> GFTDYKVADITLAAWGRRELIIAESEMPALMGLRRKYAGQQPLKGAKILGCIHMTIQTGVLIETLVALGAEVRWSSCNIFSTQDQAAAAIAAAGIPVFAWKGETEEEYEWCIEQTILKDGQPWDANMVLDDGGDLTEILHKKYPQMLERIHGITEETTTGVHRLLDMLKNGTLKVPAINVNDSVTKSKNDNKYGCRHSLNDAIKRGTDHLLSGKQALVIGYGDVGKGSSQSLRQEGMIVKVAEVDPICAMQACMDGFEVVSPYKNGINDGTEASIDAALLGKIDLIVTTTGNVNVCDANMLKALKKRAVVCNIGHFDNEIDTAFMRKNWAWEEVKPQVHKIHRTGKDGFDAHNDDYLILLAEGRLVNLGNATGHPSRIMDGSFANQVLAQIHLFEQKYADLPAAEKAKRLSVEVLPKKLDEEVALEMVKGFGGVVTQLTPKQAEYIGVSVEGPFKPDTYRY;>[3x]FTDYKVADITLAAWGRRELIIAESEMPALMGLRRKYAGQQPLKGAKILGCIHMTIQTGVLIETLVALGAEVRWSSCNIFSTQDQAAAAIAAAGIPVFAWKGETEEEYEWCIEQTILKDGQPWDANMVLDDGGDLTEILHKKYPQMLERIHGITEETTTGVHRLLDMLKNGTLKVPAINVNDSVTKSKNDNKYGCRHSLNDAIKRGTDHLLSGKQALVIGYGDVGKGSSQSLRQEGMIVKVAEVDPICAMQACMDGFEVVSPYKNGINDGTEASIDAALLGKIDLIVTTTGNVNVCDANMLKALKKRAVVCNIGHFDNEIDTAFMRKNWAWEEVKPQVHKIHRTGKDGFDAHNDDYLILLAEGRLVNLGNATGHPSRIMDGSFANQVLAQIHLFEQKYADLPAAEKAKRLSVEVLPKKLDEEVALEMVKGFGGVVTQLTPKQAEYIGVSVEGPFKPDTYRY

By hydrolyzing SAH to adenosine (Ado) and L-homocysteine (Hcy), the enzyme SAHase (SAH hydrolase) serves as an important regulator of SAM-dependent methylation through the control of the SAM:SAH ratio, and is an indicator of the biological methylation activity of the cell. SAHases are usually active as homotetramers. The protomer has a three-domain fold, with two prominent domains, the substrate- and cofactor-binding domains, separated by a deep crevice. A small C-terminal dimerization domain locks two subunits into a homodimer by quaternary complementation of the cofactor binding site, where a tightly but non-covalently bound nicotinamide adenine dinucleotide (NAD+) is found in its oxidized form.

Two complexes of Zn2+-containing PaSAHase were crystallized in the presence of K+ ions and adenosine (Ado/K+/Zn2+), or an inhibitor, 2′-deoxyadenosine (2′-dAdo/K+Zn2+). In the Zn2+-containing complexes, the divalent cation site is not fully occupied. Our crystal structures help to elucidate this puzzling behavior by showing that there is a tetrahedral zinc binding site, formed by three highly conserved amino acid residues involving S (Cys85), N (His323), and two O (Asp139) ligand atoms, located in the active site, where - together with the H323-F324 molecular gate - the divalent cation shuts access to the active site of the enzyme. Moreover, the Zn2+ cation is located at the interface between the two principal domains and is coordinated by three ligands from the substrate-binding domain (C85 Sγ, D139 O and D139 Oδ1) and one ligand from the cofactor-binding domain (H323 Nε1), thus further stabilizing the SAHaseclosed-Ligand-K+ complex. The zinc binding sites are not fully occupied and, therefore, the side chain of H323 from the molecular gate is modeled in two states, differing in ~180° flip of the imidazole ring. In both conformations the molecular gate remains shut. The rotation of the H323 side chain in the Zn2+ complex is necessary for the formation of the coordination bond. The second rotamer interacts via the H323 Nδ1 atom with the O5′ atom of adenosine. The dual conformation of H323 is correlated with a similar disorder of the adenosine O5′ atom.> IKHPIYVIQKHDASHLHYDLRLEMG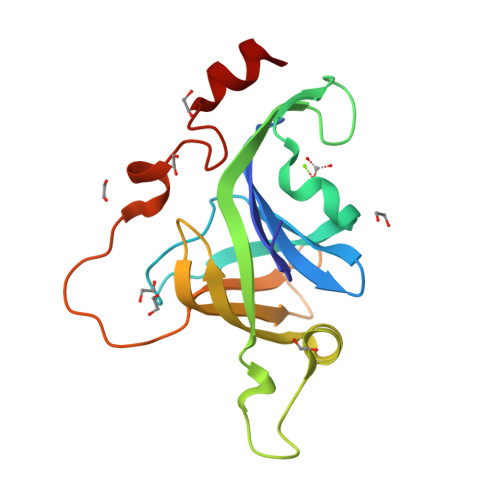GVLKSWAVPKGPSLDPKVKRLAMPTEDHPIGYATFEGVIPEGQYGGGTVMVWDIGTYRNLREEKPEGSRMTIEQSYDQGKIEVFLEGKKLKGSYALIRTGGIEKRGWLFFKMKEPHEGSYEDIEKAAPDSVLTGRTMDEIAKEG> MMQDATDPAVRAALQSQPSGLNSTDDWRQVMDRIMSLTARNPDAFRQQPQANRLSAILEAVVPARANPTHEKVLAIVNALAENRAIRPDEAGLVYDALLQRVARYNSGNVQTNLDRLVGDVREAVAQRERAQQQGNLGSMVALNAFLSTQPANVPRGQEDYTNFVSALRLMVTETPQSEVYQSGPDYFFQTSRQGLQTVNLSQAFKNLQGLWGVRAPTGDRATVSSLLTPNSRLLLLLIAPFTDSGSVSRDTYLGHLLTLYREAIGQAHVDEHTFQEITSVSRALGQEDTGSLEATLNYLLTNRRQKIPSLHSLNSEEERILRYVQQSVSLNLMRDGVTPSVALDMTARNMEPGMYASNRPFINRLMDYLHRAAAVNPEYFTNAILNPHWLPPPGFYTGGFEVPEGNDGFLWDDIDDSVFSPQPQTLLELQQREQAEAALRKESFRRPSSLSDLGAAAPRSDASSPFPSLIGSLTSTRTTRPRLLGEEEYLNNSLLQPQREKNLPPAFPNNGIESLVDKMSRWKTYAQ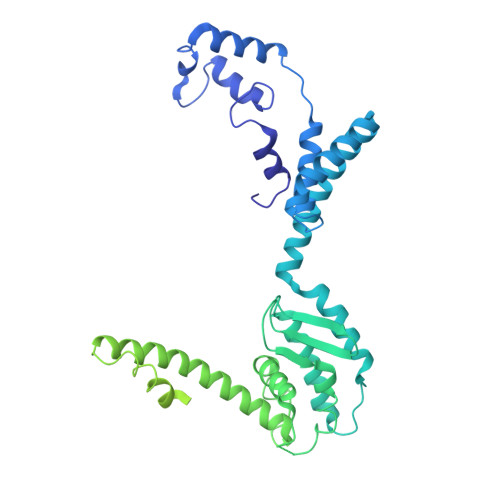EHRDVPGPRPPTRRQRHDRQRGLVWEDDDSADDSSVLDLGGSGNPFAHLRPRLGRMF> MWEQQRPRRCEAPAAPSSRPAERRAAARRSR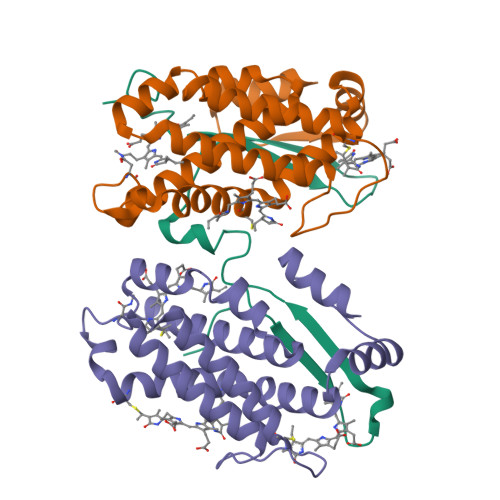AQLRMKQDDYEQWKTEFAGGFPGGEAFYKKWIEEGAKGDVPALEEELQPRSPNKKPTIYEEQMISNRGQQKGVDPTWKTLLAGGFPGGEFFFKKWIGEGAQGEVPNLDADLQPGSGSAKKTGKKEDADKSSPGGIMTPGRIMVPSGLGEEEETVDKEAPRPELYNKYFSADRLHKAPEILFEYNKTKYDRVGVRYTEVTSKASERFFPKSRMNRAPVIEISYREGAVSTASVSLSMPEISGPPALPFPVPKGDVTTTMVTDPTTGRLKLEFKVDGAAVSAYSDPRATEAYNKMIRK;>[2x]MLDAFSRVVVNSDAKAAYVGGSDLQALKSFIADGNKRLDAVNSIVSNASCMVSDAVSGMICENPGLISPGGNCYTNRRMAACLRDGEIILRYVSYALLAGDASVLEDRCLNGLKETYIALGVPTNSSIRAVSIMKAQAVAFITNTATERKMSFAAGDCTSLASEVASYFDRVGAAIS> GHMTHSAYVYQLKAVPDIFDEISQRFPDRVALIFDQRKITYRELAEQCSALAAVLQNNCLIKGDIVAIKIERSPELYIFMLALMKIGAVMVPVNSNSPERYIGEVLSAAGARYLISDDVTSVPGGAWHVLSSRTLIQNCTQQRSGNYPVLSADDPALILMTSGSTGKPKSVLIAHRGIARLGLPVPALGNSERDCYLQIADISFAASANEIWMALLTGACLTIAPPGLPDLMALARQIESDNVTMLFLSGGLFRLFVEVSVETLHIPDCVVVSGDFVNPRLFSVAVQAGKAKIFNGLGCTENSAISSLYHIQSAAALSSESPVPVGTPLPLVEMVV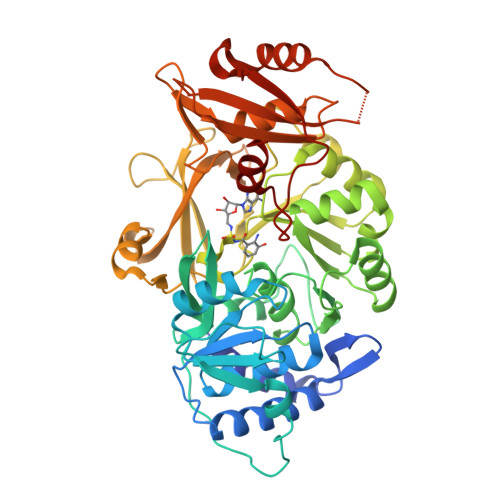FNERLQPCTCGEYGELFIAGAGVALGYSDPQLTAERFITIPYQGTDMLFYRTDDRATYDQDRNIVLVGRGNHICKIRGFRINIAGIEHLLRLHHAVEDVLIVVEETPDEPRLHACYVTQDDGLSVADLKNHLAMHAPAWMIPEKFSRLAVLPMTANGKKDRLRLKNSLLEQV>AMTDIPDRKEAVISLWPEFAKAIVSGKKTVEFRRRIPLPALSARIWIYATRPVKSVIGFAYLEAIVQGDVNTLWSRYGREAFLSEQQYRDYFEGTEKATAFLLRDHQPIRPINLDQLKEIRANFQPPQALTWLRKEETQKLVSLTS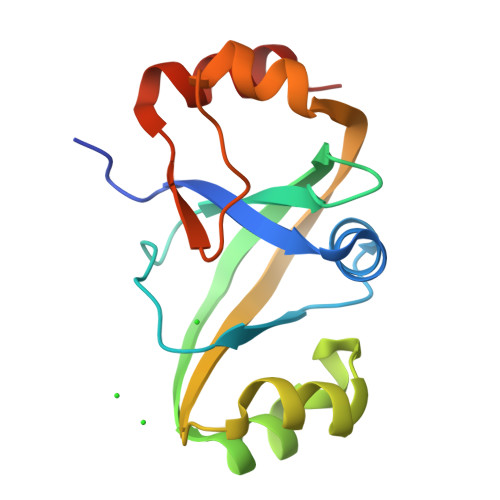QVE[2x]Enteroviruses particles are composed of single-strand RNA (virion RNA) genomes encapsulated by an icosahedral capsid of ~30 nm in diameter. In this study, we genetically perturb this equilibrium in a non-enveloped virus, enterovirus A71 to determine its structural basis. We isolate a single-point mutation variant with increased particle thermotolerance and decreased efficiency of cell entry. Using cryo-electron microscopy and molecular dynamics simulations, we determine that the thermostable native particles have acquired an expanded conformation that results in a significant increase in protein dynamics.

Particle conversion from N to empty capsids (E) follows a predetermined protein unfolding process that can be mimicked by incubating the purified N particles at high temperature. Accordingly, native particles of the WT and K162E were heated at 52 °C for 1 h to convert them to inactivated A-particle or empty E particles. Particles then were classified according to whether they had Coulomb potential at the center of the particle. A-particles showed density, but empty particles did not. The WT A- and E-particles were resolved to a resolution of 8.0 and 14 Å, respectively. The empty state WT map also matched a previously solved structure (EMDB ID: 5466) with a cross-correlation score of 0.954.

> SHSTAETTLDSFFSRAGLVGEIDLPLEGTTNPNGYANWDIDITGYAQMRRKVELFTYMRFDAEFTFVACTPTGQVVPQLLQYMFVPPGAPKPDSRESLAWQTATNPSVFVKLSDPPAQVSVPFMSPASAYQWFYDGYPTFGEHKQEKDLEYGACPNNMMGTFSVRTVGTSKSKYPLVIRIYMRMKHVRAWIPRPMRNQNYLFKANPNYAGNFIKPTGASRTAITT;> LTIGNSTITTQEAANIIVGYGEWPSYCSDTRPDVSVNRFYTLDTKLWEKSSKGWYWKFPDVLTETGVFGQNAQFHYLYRSGFCIHVQCNASKFHQGALLVAVLPEYVIGTVAGGTGTEDSHPPYKQTQPGADGFELQHPYVLDAGIPISQLTVCPHQWINLRTNNCATIIVPYINALPFDSALNHCNFGLLVVPISPLDYDQGATPVIPITITLAPMCSEFAGLRQ;> GFPTELKPGTNQFLTTDDGVSAPILPNFHPTPCIHIPGEVRNLLELCQVETILEVNNVPTNATSLMERLRFPVSAQAGKGELCAVFRADPGRSGPWQSTLLGQLCGYYTQWSGSLEVTFMFTGSFMATGKMLIAYTPPGGPLPKDRATAMLGTHVIWDFGLQSSVTLVIPTTGLVSIWYQTNYVVPIGAPNTAYIIALAAAQKNFTMQLCKDASDIL> MNLAEKMYKAGQIEFAKGNYETAIIAYT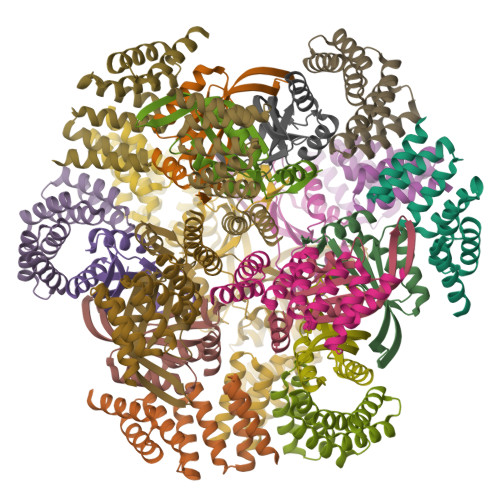LALLKDPNNAEAWYNLGEAYLALGNYEEAIEAYQKALELDPNNAEAWYNLGEAYLALGDYDNAIEAFTKALELDPNNKTAKAGLKLAKEKKALE;> MTDLSSLIETADLRLLLTTVPTETEALYLALAAVEKGLAAEVLITPVTRVRRENGKLVVEDVYRLSFKTTRERLDALVAWLQRRHPLALPECLVLTPIASSVAYRDWLRSSLQGGSHHWGGHHHHHH>MAHHHHHHMAEFSIIDQYFNRQSHPDVALGIGDDSALITPPPNQQLVICADTLVAGRHFPLETSPHAIGWKSVAVNLSDIAAMGAKPHSILLAISLPQVDHEWLEGFSQGIYDCCNQFGVALIGGDTTQGPHLTITVTAMGWIETGKAVLRSGAKVGDYVCVSGQIGDAAYGLQHLGHSLQQRLDYPTPRCKLGEELKGLASSMIDVSDGLAQDLGHILKASKVGARLILEKLPVDPVLQQIEEQQRW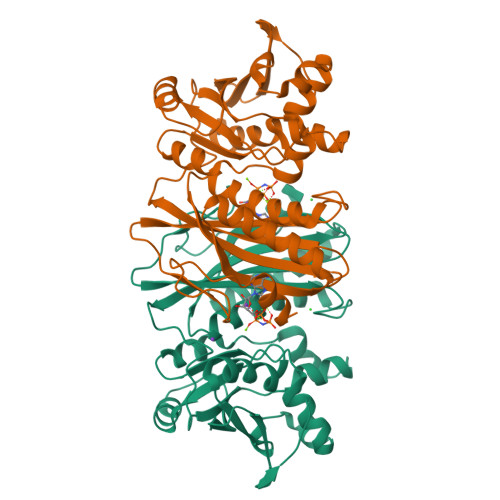QYALAGGDDYELCFTITPQNYEKLLQKQLDVKITMIGQIVEQTKLTFEHLGSDYPLQIHGYQHFA[2x]> MIRNVKKQRPVNLDLQTIRFPITAIASILHRVSGVITFVAVGILLWLLGTSLSSPEGFEQASAIMGSFFVKFIMWGILTALAYMVVVGIRHMMMDFGYLEETFEAGKRS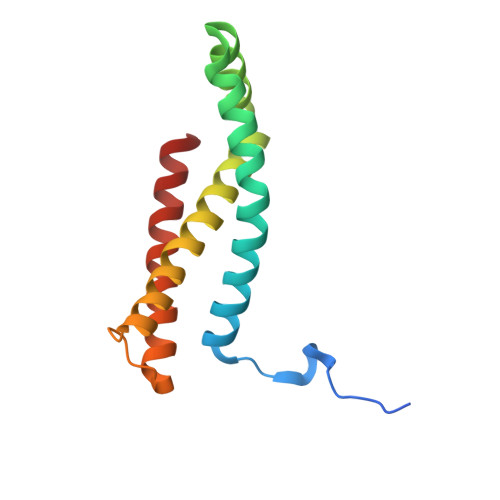AKISFVITVVLSLLAGVLVW>MRGKIYDRNGKVLAEDVERYKLVAVIDKKASANSKKPRHVVDKKETAKKLSTVINMKPEEIEKRLSQKKAFQIEFGRKGTNLTYQDKLKIEKMNLPGISLLPETERFYPNGNFASHLIGRAQKNPDTGELKGALGVEKIFDSYLSGSKGSLRYIHDIWGYIAPNTKKEKQPKRGDDVHLTIDSNIQVFVEEALDGMVERYQPKDLFAVVMDAKTGEILAYSQRPTFNPETGKDFGKKWANDLYQNTYEPGSTFKSYGLAAAIQEGAFDPDKKYKSGHRDIMGSRISDWNRVGWGEIPMSLGFTYSSNTLMMHLQDLVGADKMKSWYERFGFGKSTKGMFDGEAPGQIGWSNELQQKTSSFGQSTTVTPVQMLQAQSAFFNDGNMLKPWFVNSVENPVSKRQFYKGQKQIAGKPITKDTAEKVEKQLDLVVNSKKSHAANYRIDGYEVEGKTGTAQVAAPNGGGYVKGPNPYFVSFMGDAPKKNPKVIVYAGMSLAQKNDQEAYELGVSKAFKPIMENTLKYLNVGKSKDDTSNAEYSKVPDVEGQDKQKAIDNVSAKSLEPVTIGSGTQIKAQSIKAGNKVLPHSKVLLLTDGDLTMPDMSGWTKEDVIAFENLTNIKVNLKGSGFVSHQS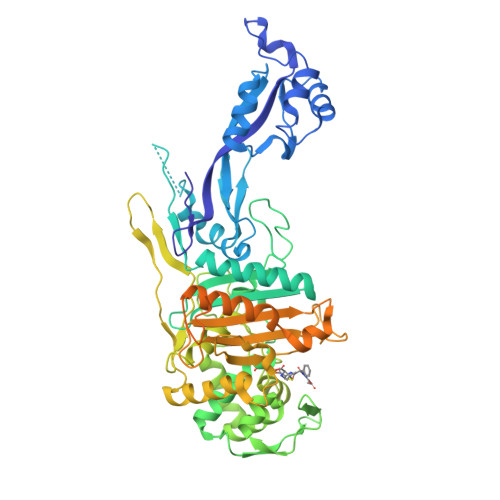ISKGQKLTEKDKIDVEFSS[2x]> ITRLQEK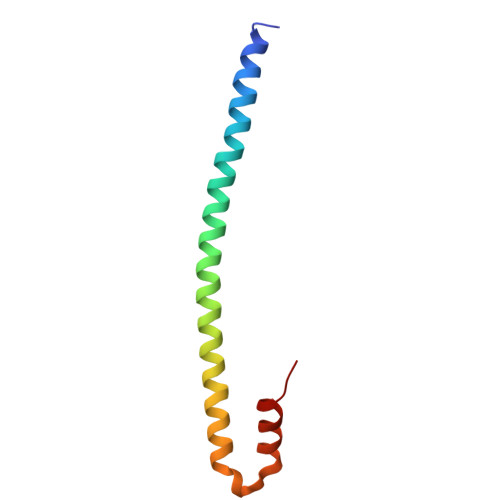EDLQELNDRLAVYIDRVRSLETENAGLRLRITESEEVVDFYFGKLRNIELICQENEGENDPVLQRIVDILYATD> GHMSLDLSVDRSSPVPLYFQLSQQLEAAIEHGALTPGSLLGNEIELAARLGLSRPTVRQAIQSLVDKGLLVRRRGVGTQVVHSKVRRPLELSSLYDDLEAAGQRPATKVLVNTVVPATAEIAAALGVAEDSEVHRIERLRLTHGEPMAYLCNYLPPGLVDLDTGQLEATGLYRLMRAAGITLHSARQSIGARAATSGEAERLGEDAGAPLLTMERTTFDDTG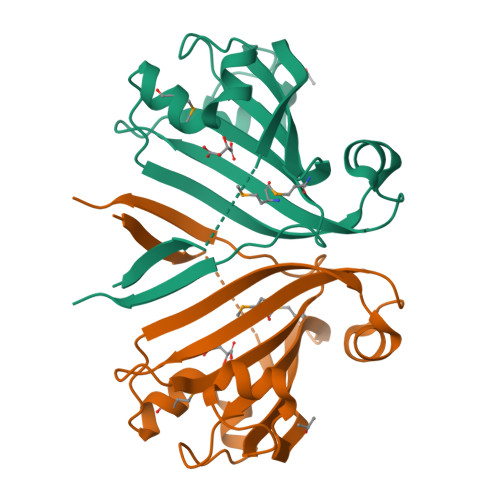RAVEFGTHTYRPSRYSFEFQLLVRP>[2x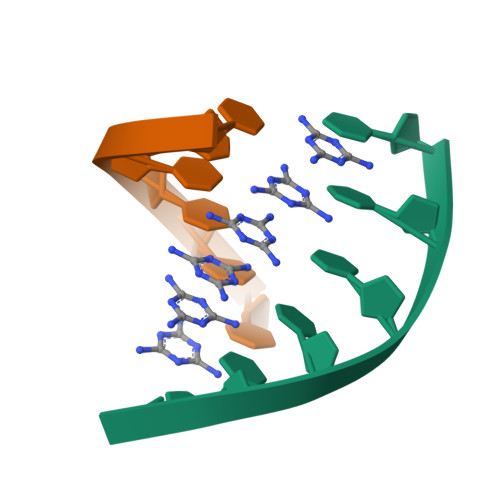]TTTTTT> GPKDNNKTLKPAIAEYIVKKAKQRIALQRWQDELNRRKNHKGMIFVENTVDLEGPPSDFYYINEYKPAPGISLVNEATFGCSCTDCFFQKCCPAEAGVLLAYNKNQQIKIPPGTPIYECNSRCQCGPDCPNRIVQKGTQYSLCIFRTSNGRGWGVKTLVKIKRMSFVMEYVGEVITSEEAERRGQFYDNKGITYLFDLDYESDEFTVDAARYGNVSHFVNHSCDPNLQVFNVFIDNLDTRLPRIALFSTRTINAGEELTFDYQMKGSGDISSDSIDHSPAKKRVRTVCKCGAVTCRGYLN

SET domain methyltransferases deposit methyl marks on specific histone tail lysine residues and play a major role in epigenetic regulation of gene transcription. HKMTs catalyze the transfer of a methyl group from the co-factor S-adenosyl-L-methionine (SAM) to a substrate lysine and, with the exception of DOT1L, are all organized around a canonical SET domain. Methylation of H3K9 in humans relies mostly on members of the Suv39 family, namely EHMT1/GLP, EHMT2/G9a, SUV39H1, SUV39H2, SETDB1 and SETDB2, as well as then non-Suv39 enzymes PRDM2 and ASH1L. Here we report the high-resolution crystal structures of the methyltransferase domains of GLP, G9a, SUV39H2 and PRDM2, and propose a structural mechanism for substrate recognition.

The Suv39 structures G9a, GLP and SUV39H2 adopt a typical fold composed of a conserved SET domain and variable I-SET insert, flanked by Pre- and Post-SET regions, and characterized by canonical features such as a pseudo-knot next to the catalytic site, distinct co-factor and substrate binding areas meeting at the site of methyl transfer, and a narrow substrate lysine docking channel. Mono-, di- or tri- methylation of H3K9 constitute distinct biochemical signals and are established by distinct histone methyltransferases; G9a and GLP are mono- and di-methylases, and SUV39H2 di- and tri-methylates a mono-methylated substrate. The Post-SET domains of G9a, GLP, SUV39H2, but not PRDM2 include a ZnCys motif previously observed in the structures of Dim-5 and the H3K4 methyltransferase MLL1. Unlike I-SET, Post-SET is absent from the PRDM2 structure, which lacks co-crystallized SAM or SAH. It is partially folded in the structures of G9a and SUV39H2 in complex with SAH and SAM respectively, and fully ordered in the ternary complexes of GLP with SAH and H3K9 peptide. As previously observed with other HKMTs (for review), the co-factor contributes to the formation of a hydrophobic, mostly aromatic cluster (composed of Post-SET Y1211/Y1154/Y261, F1215/F1158, W1216/W1159/L298, F1223/F1166/T285 and SET H1170/H1113/H220 in GLP/G9a/SUV39H2) necessary for partial folding of the Post-SET domain. Surprisingly, in our structure of SUV39H2, Post-SET Lys-264 is inserted into the partially formed substrate lysine binding channel, which may represent some form of auto-inhibitory mechanism. (2) A loose conformation when SAM or SAH, but no peptide is bound, which may also accommodate non-specific sequences.>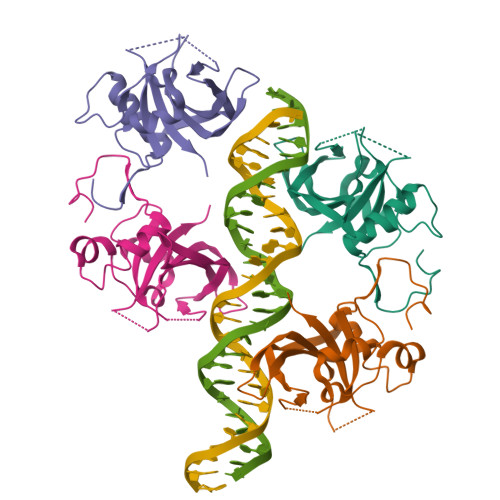[4x]HHHHHHMGIQETDPLTQLSLPPGFRFYPTDEELMVQYLCRKAAGYDFSLQLIAEIDLYKFDPWVLPNKALFGEKEWYFFSPRDRKYPNGSRPNRVAGSGYWKATGTDKIISTEGQRVGIKKALVFYIGKAPKGTKTNWIMHEYRLIEPSRRNGSTKLDDWVLCRIYKKQSSAQK> MTFELKRVALPNGIHLDVVDEGPTDAPVLIFLHGFPESHRTWRHQIRHFSDRFRCIAPDQRGYRGSSKPQEVAAYTPDKLIGDIFLLADTLGIGSFTIVGHDWGGAIAWGVALGGQHLRVERAIIANAPHPAIFQKLLYTHPVQREASQYIRGFRDPANDALVKEHGLTGLLMKEVKWDRPSAMEPEERDQLLRDWQNHDAAFGMLNYYRASPIDVPTMDAPFKVPAGYTPPQLPRLTIPTLVIWALDDLALPPENLEGLEEIIDPLTIVRVPDCGHFVPWEAPDAVNAAMEGFLAGHHHHHH

Epoxide hydrolases (EHs, EC 3.3.2.9) are enzymes that catalyze the in vivo hydrolysis of an epoxide ring to the corresponding vicinal diols. Two novel EH enzymes of the α/β fold class have been identified from metagenomic samples from diverse locations in Russia and China. The nucleophile Asp102 in Sibe-EH (Asp101 in CH65-EH), is complemented by His277 and Asp249 (His270 and Asp241) to form a catalytic triad.

The ORF found in the Russian metagenome (Sibe-eh) is 891 nt long and encodes for a protein (Sibe-EH) of 297 amino acids that has 30% identity with the CH65-EH protein sequence. Sibe-EH is monomeric in the crystal structure and in solution which is similar to many other bacterial EHs and plant, such as potato, EHs. All residues of Sibe-EH plus one His residue belonging to the C-terminal His tag have been modeled into the electron density. The amino acids Pro36 and Pro266 are in the cis- conformation in the Sibe-EH structure. The Sibe-EH was active on all tested substrates resulting in conversions > 99% for substrates (2), (5), and (6), around 90% for substrates (3) and (4), and around 40% for substrate (1). Sibe-EH displayed an optimum temperature at 30°C and retained more than 40% of activity at 40°C, while CH65-EH showed the highest activity at temperatures around 50°C and retained more than 60% of activity at 70°C. The substrate epoxide oxygen binds to the side chain hydroxyls of Tyr150 and Tyr209 in Sibe-EH, and its likely position is marked by a conserved water molecule interacting with these residues. In the case of CH65-EH and Sibe-EH the entrance to the active site cavity as seen in B. megaterium EH is totally obstructed by the adjacent monomer in the CH65-EH dimer and by a very different conformation in Sibe-EH in the region of residues 159–180. The high ee observed for the meso-epoxide in the Sibe-EH reaction can be explained by the formation of favorable protein-ligand hydrophobic interactions when the ligand is attacked at the (S)-carbon to release the (R, R) product.Phytoplankton blooms produce large quantities of beta-glucans, such as laminarin, a soluble β-1,3-glucan with β-1,6 side chains. We cloned and examined the genes encoding FbGH17A (locus tag: FORMB_24720), FaGH17B (locus tag: FORMB_24740), and FbGH30 (locus tag: FORMB_24730). The data indicated an enzymatic functional cascade in three steps: The exo-acting β-1, 6-glucosidase FbGH30 removes the glucose side chains from laminarin. The endo-acting β-1, 3-glucan hydrolase FbGH17A degrades the remaining debranched laminarin into oligosaccharides.

The enzyme FbGH17A hydrolyzed both the debranched laminarin product of FbGH30 and the native laminarin, although with a markedly higher specific activity on the debranched product (KM: 1.6 ± 0.1 mM; Kcat/KM: 36056 M−1s−1) than on laminarin itself (KM: 4.3 ± 0.1 mM; Kcat/KM: 25744 M−1s−1). In order to examine the molecular basis of substrate specificity the X-ray crystal structure of GH17A was solved. Compared to the monomeric GH17 structures, FbGH17A has significant insertions and is larger. The structure of GH17A allows for the deduction of the molecular basis of substrate specificity for the laminarinase. Based on the GH17 complexes obtained for R. miehei, a model was generated of a laminarin product involving five monomers bound to the catalytic groove, two on the aglycone side, and three on the glycone side. The reducing and non-reducing ends of the modeled glycan are free, suggesting the protein can act in the middle of the chain as expected for an endo-acting glycoside hydrolase. Furthermore, given the conformation of the modeled glycan, 6-O-β-glucose branching would be possible only at subsite + 1 and anything further away (+ 3 or − 4). In other words, within the native polysaccharide the enzyme would need a stretch of at least three free β1,3-glucose moieties to act. This structural data supports the observation that GH17 activity on laminarin is bolstered by the action of the debranching enzyme GH30. Here, two enzymes that are likely residents of the periplasm are shown to work together towards the complete degradation of laminarin in a highly specific manner. The X-ray crystal structure of GH17A reveals the possible molecular determinants of substrate specificity and the propensity of the enzyme to be more active on unbranched laminarin.

>[6x]MRATKHILILILLVFLVISCKNKQSNTQNPNQQNQNEVTAKDILGNSKYLAISYGGYRKKSRDFQPSIEELKEDMKILHAMNIRILRTYNVRLAHTSNILKAIRELKNEDANFEMYMMVGAWIDCKNAWTDQPLNHHEESENNASEIDRAVALAQEFPDIVKVIAVGNEAMVKWAASYFVQPAVILKWVNHLQALKKKGDLSKDLWITSSDNFASWGGGDPQYHVEDLTKLIEAVDYLSVHTYPMHDTHYNPIFWGVFGDETELSSLKRIDIAMNRAKTYAVSQSDSVASYIKSLGINKPIHIGETGWASFSNGYYGAKGSKATDEYKEAIFYNHIREWTNEANMSCFYFEAFDEPWKDAHNSGGSENHFGLFTVDGKAKYVLWDLVDKGVFEGLTRGGNPITKTYNGNKEALFLEVELPPVKKEITKNH> MTGYLTIGGQRYQAEINDLENLGEMGSGTCGQVWKMRFRKTGHVIAVKQMRRSGNKEENKRILMDLDVVLKSHDCPYIVQCFGTFITNTDVFIAMELMGTCAEKLKKRMQGPIPERILGKMTVAIVKALYYLKEKHGVIHRDVKPSNILLDERGQIKLCDFGISGRLVDSKAKTRSAGCAAYMAPERIDPPDPTKPDYDIRADVWSLGISLVELATGQFPYKNCKTDFEVLTKVLQEEPPLLPGHMGFSGDFQSFVKDCLTKDHRKRPKYNKLLEHSFIKRYETLEVDVAS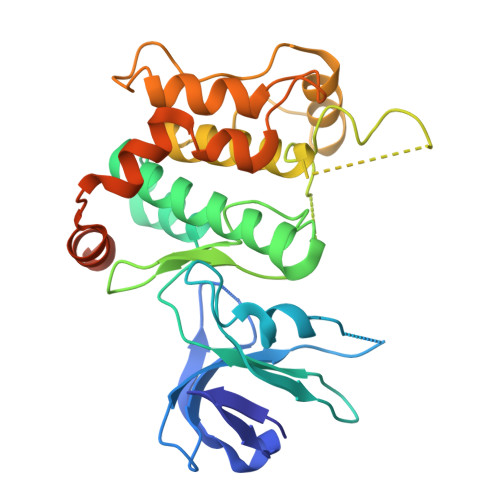WFKDVMAKTESPRTSGVLSQPHLPFFRHHHHHH>SDVLHPYRDLFPQIGQRVMIDDSSVVIGDVRLADDVGIWPLVVIRGDVHYVQIGARTNIQDGSMLHVTHKSSYNPDGNPLTIGEDVTVGHKVMLHGCTIGNRVLVGMGSILLDGAIVEDDVMIGAGSLVPQNKRLE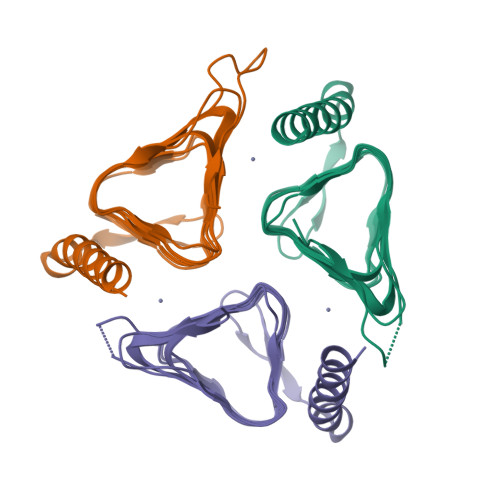SGYLYLGSPVKQIRPLSDEEKAGLRYSANNYVKWKDEYLDQGNQTQP[3x]>[2x]STRSPRPFNEIPSPGDNGWLNLYHFWRETGTHKVHLHHVQNFQKYGPIYREKLGNVESVYVIDPEDVALLFKSEGPNPERFLIPPWVAYHQYYQRPIGVLLKKSAAWKKDRVALNQEVMAPEATKNFLPLLDAVSRDFVSVLHRRIKKAGSGNYSGDISDDLFRFAFESITNVIFGERQGMLEEVVNPEAQRFIDAIYQMFHTSVPMLNLPPDLFRLFRTKTWKDHVAAWDVIFSKADIYTQNFYWELRQKGSVHHDYRGILYRLLGDSKMSFEDIKANVTEMLAGGVDTTSMTLQWHLYEMARNLKVQDMLRAEVLAARHQAQGDMATMLQLVPLLKASIKETLRLHPISVTLQRYLVNDLVLRDYMIPAKTLVQVAIYALGREPTFFFDPENFDPTRWLSKDKNITYFRNLGFGWGVRQCLGRRIAELEMTIFLINMLENFRVEIQHLSDVGTTFNL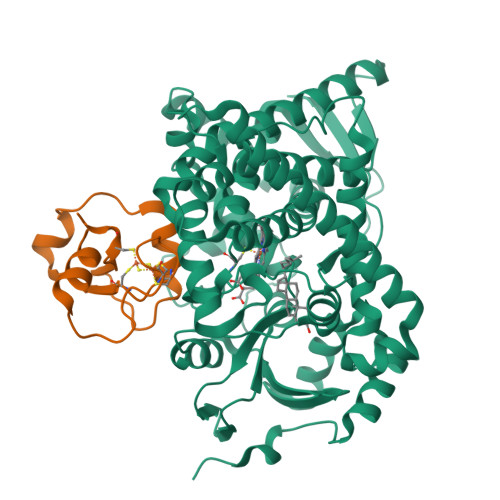ILMPEKPISFTFWPFNQEATQQHHHHHH;>[2x]SSEDKITVHFINRDGETLTTKGKVGDSLLDVVVENNLDIDGFGACEGTLACSTCHLIFEDHIYEKLDAITDEENDMLDLAYGLTDRSRLGCQICLTKSMDNMTVRVPETVADAR> MGPFYGGYNVIALDREYRHALVCGPDRDYLWINSRTPTISDEVKQ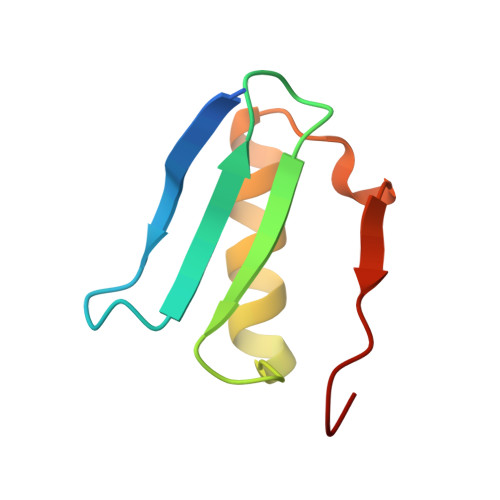EMLAVATREGFDVSKFIWVQQPGS>[6x]MSLYRLIFSSQGIPNLQPQDLKDILESSQRNNPANGITGLLCYSKPAFLQVLEGECEQVNETYHRIVQDERHHSPQIIECMPIR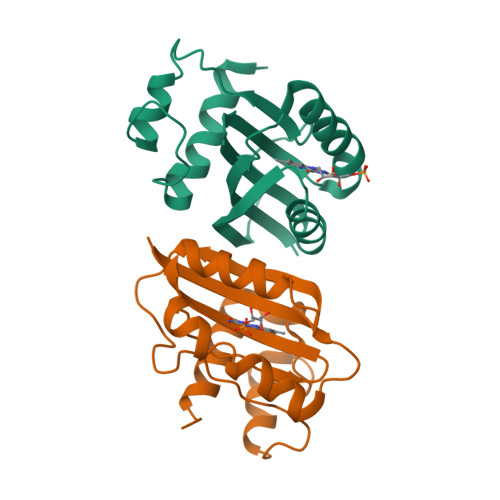RRNFEVWSMQAITVNDLSTEQVKTLVLKYSGFTTLRPSAMDPEQCLNFLLDIAKIYELSDNFFLDL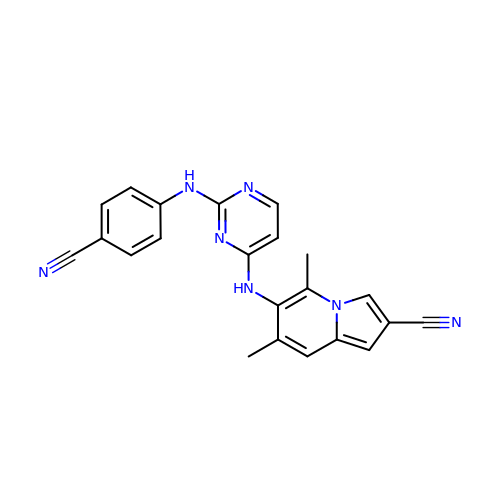(4R)-6-{[2-(4-cyanoanilino)pyrimidin-4-yl]amino}-5,7-dimethylindolizine-2-carbonitrile | C22 H17 N7 | GMFRQOLPQYTHQH-UHFFFAOYSA-N> GSGPPGPPGPPGPPGARGQAGVMGFPGPPGPPGPPGRAPTDQHIKQVCMRVIQEHFAEMAASLKRPDSGAT;> GSGPPGPPGPPGPPGARGEPGNIGFPGPPGPPGPPGRDATDQHIVDVALKMLQEQLAEVAVSAKREALGAV;> GSGPPGPPGPPGPPGARGQAGVMGFPGPPGPPGPPGKEASEQRIRELCGGMISEQIAQLAAHLRKPLAPGSI

Two host-guest collagen peptides (GPP)4-(GXY)4-(GPP)3, where (GXY)4 sequences are from the α1 and α2 chains of human type I collagen, were recombinantly linked to chains A, B and C (corresponding to α1, α2 and α3 in collagen nomenclature and omitted here to avoid confusion) of the NC2 domain in the following combinations designated as α1Aα1Bα1C (for short 111), α1Aα1Bα2C (112), α1Aα2Bα1C (121), α2Aα1Bα1C (211) and α2Aα2Bα2C (222). Three unique chains form a parallel α-helical right-handed bundle. The most important observation is that the triple-helical chain stagger is entirely determined by the NC2 domain.

All five constructs were screened for crystallization, but only three of them yielded crystals of sufficient quality, crystal structures for 111, 211 and 121 were independently solved using the MAD phasing from selenomethionine derivatives (thereafter designated as 111sm, 211sm and 121sm) to 2.25 Å, 2.10 Å and 1.6 Å, respectively. Whereas the crystal packing for 111sm and 211sm are similar (two trimers per asymmetric unit), it differs from that for 121nat or 121sm (one trimer per asymmetric unit). An overall superimposition of 121nat and 121sm (r.m.s.d. of 0.35 Å) confirmed the identity of the two structures. The most deviated pair is the first trimer (chains A, B, C in the asymmetric unit) of 121sm versus the second trimer (chains D, E, F) of 111sm (r.m.s.d. of 3.01 Å). On the other hand, superimposition within the NC2 domain demonstrated high identity of the trimerization domain and adjacent residues within the triple-helical portion. Most of deviations observed for overall superimposition of trimers are attributed to distal flexibility of the triple helical fragments caused by crystal packing (Fig. 2A vs B). Namely, a triple helical chain linked to chain B of the NC2 domain is always in the leading position, the one linked to A is in the middle, and the third one linked to C is in the trailing position. We suggest here to use a rule of BAC-translation: chain B is leading, A is middle, C is trailing. This way, construct 121 (or α1Aα2Bα1 C) translates into staggering order of α2α1α1, whereas 211 translates into α1α2α1. Despite the variations of composition (homo-trimeric for 111) and stagger (121 or 211) that might not represent a native stagger, the regions of sequences derived from type I collagen are well structured. Crystal structures of 111, 121 and 211 constructs demonstrated that a staggering order can be manipulated at least for short native collagenous sequences, meaning that such sequences are rather adaptive to various abnormal conformations.> MGSDKIHHHHHHMRILSGMRPTGKLHIGHLVGALENWVKLQEEGNECFYFVADWHALTTHYDDVSKLKEYTRDLVRGFLACGIDPEKSVIFVQSGVKEHAELALL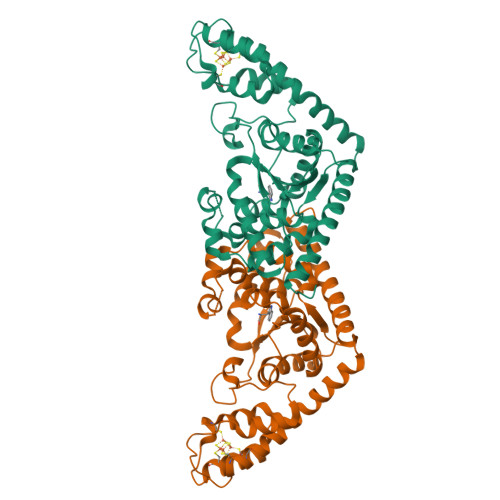FSMIVSVSRLERVPTYKEIKSELNYKDLSTAGFLIYPVLQAADILIYKAEGVPVGEDQVYHIELTREIARRFNYLYDEVFPEPEAILSRVPKLPGTDGRKMSKSYGNIINLEISEKELEQTILRMMTDPARVRRSDPGNPENCPVWKYHQAFDISEEESKWVWEGCTTASIGCVDCKKLLLKNMKRKLAPIWENFRKIDEDPHYVDDVIMEGTKKAREVAAKTMEEVRRAMNLMF>[6x]GAMGVKKVFTADQLKVAWGDADYELADGQWKLSFAKQYNQVK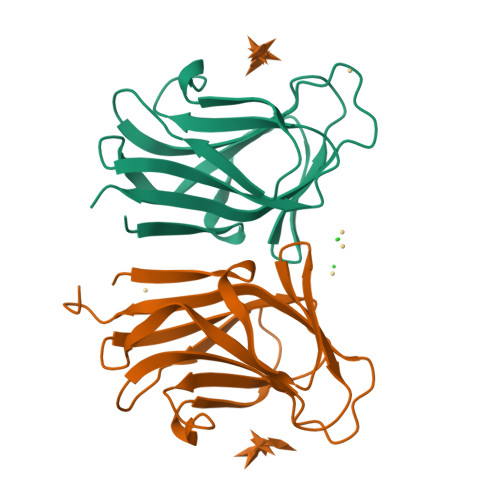WTLPESIEMSQVNAVTFQVADQKVPISLKVYNGGDDATAANTQYGLSGQTEYTINPSGDGAIDAVGIMITEDKPENATVSLVSVTFELKAGAGDAKLGD> MLGSLVLRRKALAPRLLLRLLRSPTLRGHGGASGRNVTTGSLGEPQWLRVATGGRPGTSPALFSGRGAATGGRQGGRFDTKCLAAATWGRLPGPEETLPGQDSWNGVPSRAGLGMCALAAALVVHCYSKSPSNKDAALLEAARANNMQEVSRLLSEGADVNAKHRLGWTALMVA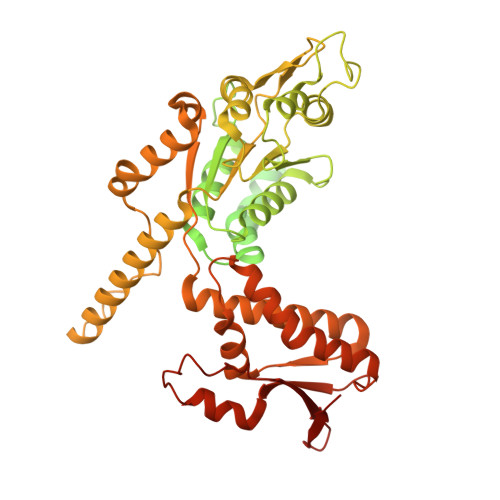AINRNNSVVQVLLAAGADPNLGDDFSSVYKTAKEQGIHSLEVLITREDDFNNRLNNRASFKGCTALHYAVLADDYRTVKELLDGGANPLQRNEMGHTPLDYAREGEVMKLLRTSEAKYQEKQRKREAEERRRFPLEQRLKEHIIGQESAIATVGAAIRRKENGWYDEEHPLVFLFLGSSGIGKTELAKQTAKYMHKDAKKGFIRLDMSEFQERHEVAKFIGSPPGYVGHEEGGQLTKKLKQCPNAVVLFDQVDKAHPDVLTIMLQLFDEGRLTDGKGKTIDCKDAIFIMTSNVASDEIAQHALQLRQEALEMSRNRIAENLGDVQISDKITISKNFKENVIRPILKAHFRRDEFLGRINEIVYFLPFCHSELIQLVNKELNFWAKRAKQRHNITLLWDREVADVLVDGYNVHYGARSIKHEVERRVVNQLAAAYEQDLLPGGCTLRITVEDSDKQLLKSPELPSPQAEKRLPKLRLEIIDKDSKTRRLDIRAPLHPEKVCNTI> G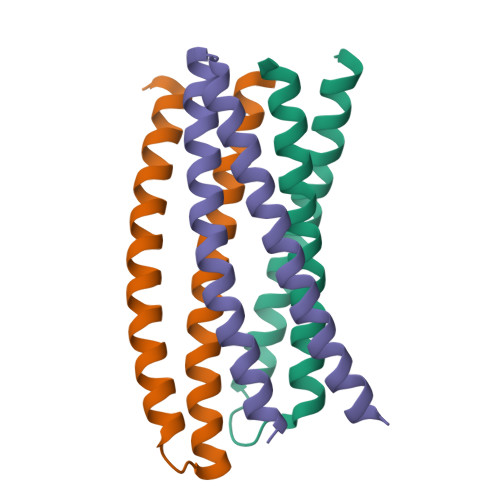SSPEEEKLKELLKELKKVLDRLKKILERNDEEIKKSDELDDESLLEDIVELLKEIIKLWKILVELSDILLKLIS;> SSPVDEIDKEVKKLEEEAKKSQEEVERLKQEVEKASKAGLDHEGDSRIFKKIHDVVTKQIKVIIRLIEVYVRLVEIIL;> GSKQKEAIKVYLELLEVHSRVLKALIEQIKLFIELIKRPDEDLADKVRKSSEELKKIIKEVEKILRKVDDILYKVKS> MNNGEGEVMDLRDIDLNLLVVFNQLLLDRSVSTAGEK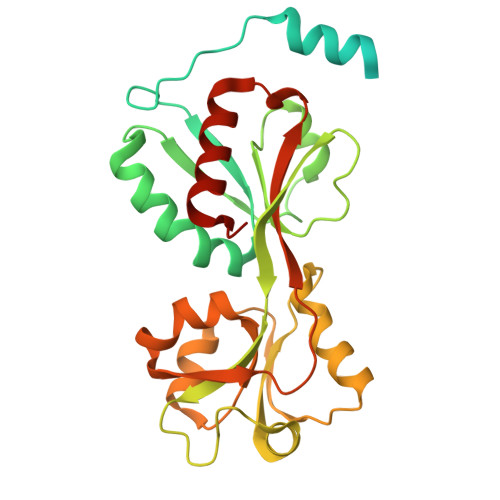LGLTQPAVSNSLKRLRTALNDDLFLRTSKGMEPTPYALHLAEPVIYALNTLQTALTTRDSFDPFASTRTFNLAMTDIGEMYFMPPLMEALAQRAPHIQISTLRPNAGNLSEDMESGAVDLALGLLPELQTGFFQRRLFRHRYVCMFRKDHPSAKSPMSLKQFSELEHVGVVALNTGHGEVDGLLERAGIKRRMRLVVPHFIAIGPILHSTDLIATVPERFAVRCEVPFGLTTSPHPAKLPDIAINLFWHAKYNRDPGNMWLRQLFVELFSEAHHHHHH>[6x]GPGYQMESNGVPMITLSSGIRMPALGMGTAETMVKGTEREKLAFLKAIEVGYRHFDTAAAYQSEECLGEAIAEALQLGLIKSRDELFITSKLWCADAHADLVLPALQNSLRNLKLDYLDLYLIHHPVSLKPGKFVNEIPKDHILPMDYKSVWAAMEECQTLGFTRAIGVCNFSCKKLQELMAAAKIPPVVNQVEMSPTLHQK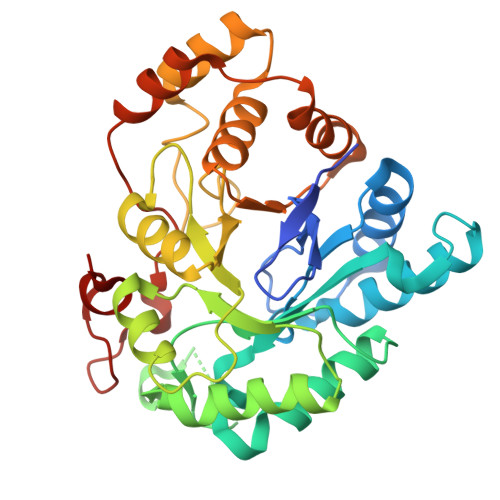NLREYCKANNIMITAHSVLGAICAPWGSNAVMDSKVLHQIAVARGKSVAQVSMRWVYQQGASLVVKSFNEGRMKENLKIFDWELTAENMEKISEIPQSRTSSADFLLSPTGPFKTEEEFWDEKD> SVATVSES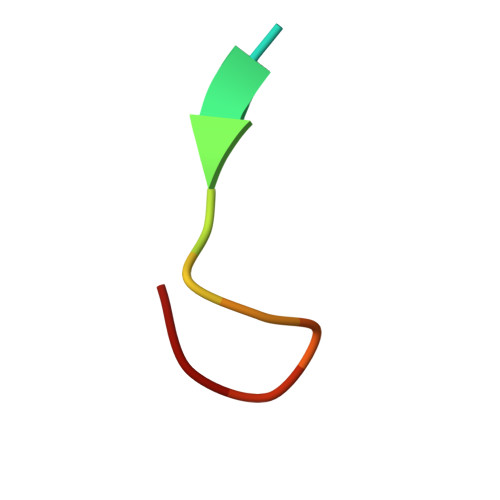FLTE> MAYIAVPAVVDSRSSEAIGLLESFGVDAGADANDVSYQDHDYVLDQLQYMLDGYEAGDVIDALVHKNWLHHSVYCLLPPKSQLLEYWKSNPSAIPDNVDRRLRKRLMLKKDLRKDDEYNQLARAFKISDVYAPLISSTTSPMTMIQNLNQGEIVYTTTDRVIGARILLYAPRKYYASTLSFTMTKCIIPFGKEVGRVPHSRFNVGTFPSIATPKCFVMSGVDIESIPNEFIKLFYQRVKSVHANILNDISPQIVSDMINRKRLRVHTPSDRRAAQLMHLPYHVKRGASHVDVYKVDVVDMLFEVVDVADGLRNVSRKLTMHTVPVCILEMLGIEIADYCIRQEDGMLTDWFLLLTMLSDGLTDRRTHCQYLINPSSVPPDVILNISITGFINRHTIDVMPDIYDFVKPIGAVLPKGSFKSTIMRVLDSISILGIQIMPRAHVVDSDEVGEQMEPTFEQAVMEIYKGIAGVDSLDDLIKWVLNSDLIPHDDRLGQLFQAFLPLAKDLLAPMARKFYDNSMSEGRLLTFA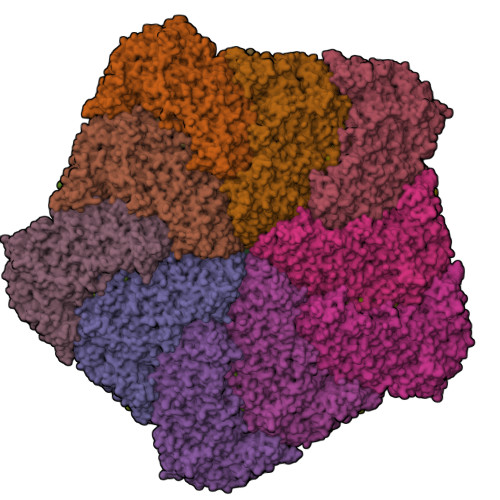HADSELLNANYFGHLLRLKIPYITEVNLMIRKNREGGELFQLVLSYLYKMYATSAQPKWFGSLLRLLICPWLHMEKLIGEADPASTSAEIGWHIPREQLMQDGWCGCEDGFIPYVSIRAPRLVIEELMEKNWGQYHAQVIVTDQLVVGEPRRVSAKAVIKGNHLPVKLVSRFACFTLTAKYEMRLSCGHSTGRGAAYSARLAFRSDLA;> MSSMILTQFGPFIESISGITDQSNDVFEDAAKAFSMFTRSDVYKALDEIPFSDDAMLPIPPTIYTKPSHDSYYYIDALNRVRRKTYQGPDDVYVPNCSIVELLEPHETLTSYGRLSEAIENRAKDGDSQARIATTYGRIAESQARQIKAPLEKFVLALLVAEAGGSLYDPVLQKYDEIPDLSHNCPLWCFREICRHISGPLPDRAPYLYLSAGVFWLMSPRMTSAIPPLLSDLVNLAILQQTAGLDPSLVKLGVQICLHAAASSSYAWFILKTKSIFPQNTLHSMYESLEGGYCPNLEWLEPRSDYKFMYMGVMPLSAKYARSAPSNDKKARELGEKYGLSSVVGELRKRTKTYVKHDFASVRYIRDAMACTSGIFLVRTPTETVLQEYTQSPEIKVPIPQKDWTGPIGEIRILKDTTSSIARYLYRTWYLAAARMAAQPRTWDPLFQAIMRSQYVTARGGSGAALRESLYAINVSLPDFKGLPVKAATKIFQAAQLANLPFSHTSVAILADTSMGLRNQVQRRPRSIMPLNVPQQQVSAPHTLTADYINYHMNLSTTSGSAVIEKVIPLGVYASSPPNQSINIDISACDASITWDFFLSVIMAAIHEGVASSSIGKPFMGVPASIVNDESVVGVRAARPISGMQNMIQHLSKLYKRGFSYRVNDSFSPGNDFTHMTTTFPSGSTATSTEHTANNSTMMETFLTVWGPEHTDDPDVLRLMKSLTIQRNYVCQGDDGLMIIDGTTAGKVNSETIQKMLELISKYGEEFGWKYDIAYDGTAEYLKLYFIFGCRIPNLSRHPIVGKERANSSAEEPWPAILDQIMGVFFNGVHDGLQWQRWIRYSWALCCAFSRQRTMIGESVGYLQYPMWSFVYWGLPLVKAFGSDPWIFSWYMPTGDLGMYSWISLIRPLMTRWMVANGYVTDRCSPVFGNADYRRCFNELKLYQGYYMAQLPRNPKKSGRAAPREVREQFTQALSDYLMQNPELKSRVLRGRSEWEKYGAGIIHNPPSLFDVPHKWYQGAQEAAIATREELAEMDETLMRARRHSYSSFSKLLEAYLLVKWRMCEAREPSVDLRLPLCAGIDPLNSDPFLKMVSVGPMLQSTRKYFAQTLFMAKTVSGLDVNAIDSALLRLRTLGADKKALTAQLLMVGLQESEADALAGKIMLQDVNTVQLARVVNLAVPDTWMSLDFDSMFKHHVKLLPKDGRHLNTDIPPRMGWLRAILRFLGAGMVMTATGVAVDIYLEDIHGGGRSLGQRFMTWMRQEGRSA;>YQCHVCSAVLFSPLDLDAHVASHGLHGNMTLTSSDIQRHITEFISSWQNHPIVQVSADVENKKTAQLLHADTPRLVTWDAGLCTSFKIVPIVPAQVPQDVLAYTFFTSSYAIQSPFPEAAVSRIVVHTRWASNVDFDRDSSVIMAPPTENNIHLFKQLLNTETLSVRGANPLMFRANVLHMLLEFVLDNLYLNRHTGFSQDHTPFTEGANLRSLPGPDAEKWYSIMYPTRMGTPNVSKICNFVASCVRNRVGRFDRAQMMNGAMSEWVDVFETSDALTVSIRGRWMARLARMNINPTEIEWALTECAQGYVTVTSPYAPSVNRLMPYRISNAERQISQIIRIMNIGNNATVIQPVLQDISVLLQRISPLQIDPTIISNTMSTVSESTTQTLSPASSILGKLRPSNSDFSSFRVALAGWLYNGVVTTVIDDSSYPKDGGSVTSLENLWDFFILALALPLTTDPCAPVKAFMTLANMMVGFETIPMDNQIYTQSRRASAFSTPHTWPRCFMNIQLISPIDAPILRQWAEIIHRYWPNPSQIRYGAPNVFGSANLFTPPEVLLLPIDHQPANVTTPTLDFTNELTNWRARVCELMKNLVDNQRYQPGWTQSLVSSMRGTLDKLKLIKSMTPMYLQQLAPVELAVIAPMLPFPPFQVPYVRLDRDRVPTMVGVTRQSRDTITQPALSLSTTNTTVGVPLALDARAITVALLSGKYPPDLVTNVWYADAIYPMYADTEVFSNLQRDMITCEAVQTLVTLVAQISETQYPVDRYLDWIPSLRASAATAATFAEWVNTSMKTAFDLSDMLLEPLLSGDPRMTQLAIQYQQYNGRTFNIIPEMPGSVIADCVQLTAEVFNHEYNLFGIARGDIIIGRVQSTHLWSPLAPPPDLVFDRDTPGVHIFGRDCRISFGMNGAAPMIRDETGLMVPFEGNWIFPLALWQMNTRYFNQQFDAWIKTGELRIRIEMGAYPYMLHYYDPRQYANAWNLTSAWLEEITPTSIPSVPFMVPISSDHDISSAPAVQYIISTEYNDRSLFCTNSSSPQTIAGPDKHIPVERYNILTNPDAPPTQIQLPEVVDLYNVVTRYAYETPPITAVVMGVP[10x];>[5x]MKRIPRKTKGKSSGKGNDSTERADDGSSQLRDKQNNKAGPATTEPGTSNREQYKARPGIASVQRATESAEMPMKNNDEGTPDKKGNTKGDLVNEHSEAKDEADEATKKQAKDTDKSKAQVTYSDTGINNANELSRSGNVDNEGGSNQKPMSTRIAEATSAIVSKHPARVGLPPTASSGHG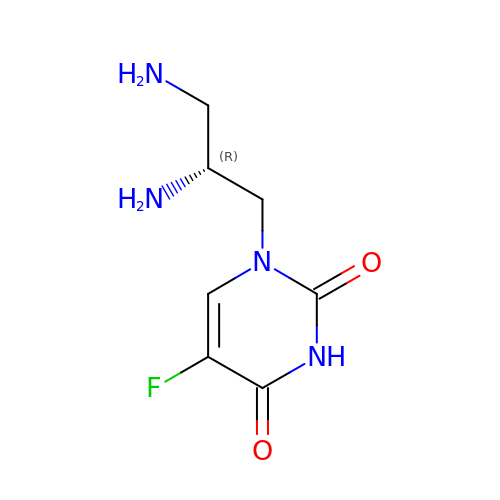1-[(2R)-2,3-diaminopropyl]-5-fluoropyrimidine-2,4(1H,3H)-dione | C7 H11 F N4 O2 | ZBKWVMMCABYTAU-SCSAIBSYSA-N> MGSSHHHHHHSSGRENLYFQGMATITLERDGLQLVGTREEPFGEIYDMAIIFHGFTANRNTSLLREIANSLRDENIASVRFDFNGHGDSDGKFENMTVLNEIEDANAILNYVKTDPHVRNIYLVGHAQGGVVASMLAGLYPDLIKKVVLLAPAATLKGDALEGNTQGVTYNPDHIPDRLPFKDLTLGGFYLRIAQQLPIYEVSAQFTKPVCLIHGTDDTVVSPNASKKYDQIYQNSTLHLIEGADHCFSDSYQKNAVNLTTDFLQ

We previously showed that LJ0536, a cinnamoyl esterase purified from L. johnsonii N6.2, is active towards a variety of substrates including short acyl chain aliphatic esters and phenolic esters. The structure showed a canonical α/β fold characteristic of esterases, and the enzyme is dimeric. Two classical serine esterase motifs (GlyXSerXGly) can be recognized from the amino acid sequence, and the structure revealed that the catalytic triad of the enzyme is formed by Ser106, His225, and Asp197, while the other motif is non-functional. The structure revealed a prominent inserted α/β subdomain of 54 amino acids, from which multiple contacts to the aromatic acyl groups of the substrates are made.

The Ser106Ala-ethyl ferulate complex crystallized in two forms (Form I and Form II with a dimer and a single chain in the asymmetric units, respectively). The two ethyl ferulate crystal forms are nearly identical in structure. We focused our analysis on Form II due to better occupancy of the ligand in the active site. The electron density for the C2 atom of ethyl ferulate has missing electron density in our structure, which is consistent with this atom being part of the leaving group after hydrolysis. One oxygen atom of the carbonyl group that forms the ester interacts directly with the oxyanion hole formed by the backbone nitrogen atoms of Phe34 and Gln107, while the other oxygen interacts with His225 and an ordered water molecule present in the caffeic and ferulic acid structures (the ethoxy group of ethyl ferulate occupies the space of this water molecule). Due to these interactions, ethyl ferulate rotates slightly and positions the ester bond perpendicular to Ser106 at a distance of 2.73 Å. The ester bond is strained from planarity (bond angle of 116°), suggesting that the hydrolytic mechanism involves a tetrahedral enzyme-ester intermediate, typical of esterases. We observed a water molecule 3.3 Å from the non-carbonyl oxygen of the ester bond of ethyl ferulate towards the solvent-exposed face of the pocket. It is possible that this corresponds to the water molecule that is the target for deprotonation by His225 to hydrolyze the tetrahedral intermediate between the ligand and Ser106, regenerating the enzyme and releasing the product. The opposite end of the ligands, on the far side of the ester moiety, such as the ethoxyl group of ethyl ferulate, rests on a more solvent-exposed area of the groove and has few interactions with the protein.> SDRVYIHPFHLVIHNESTCEQLAKANAGKPKDPTFIPAPIQAKTSPVDEKALQDQLVLVAAKLDTEDKLRAAMVGMLANFLGFRIYGMHSELWGVVHGATVLSPTAVFGTLASLYLGALDHTADRLQAILGVPWKDKNCTSRLDAHKVLSALQAVQGLLVAQGRADSQAQLLLSTVVGVFTAPGLHLKQPFVQGLALYTPVVLPRSLDFTELD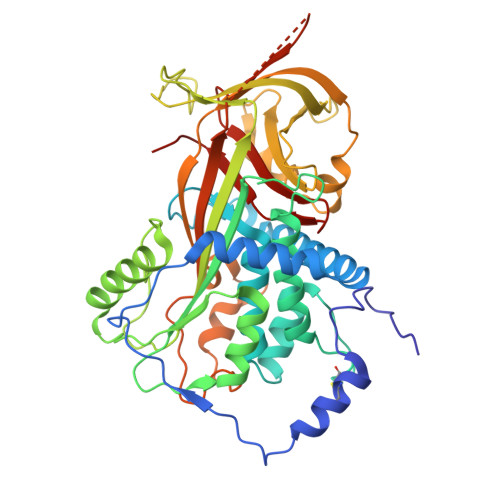VAAEKIDRFMQAVTGWKTGCSLMGASVDSTLAFNTYVHFQGKMKGFSLLAEPQEFWVDNSTSVSVPMLSGMGTFQHWSDIQDNFSVTQVPFTESACLLLIQPHYASDLDKVEGLTFQQNSLNWMKKLSPRTIHLTMPQLVLQGSYDLQDLLAQAELPAILHTELNLQKLSNDRIRVGEVLNSIFFELEADEREPTESTQQLNKPEVLEVTLNRPFLFAVYDQSATALHFLGRVANPLSTA> GPSQPTYPGDDAP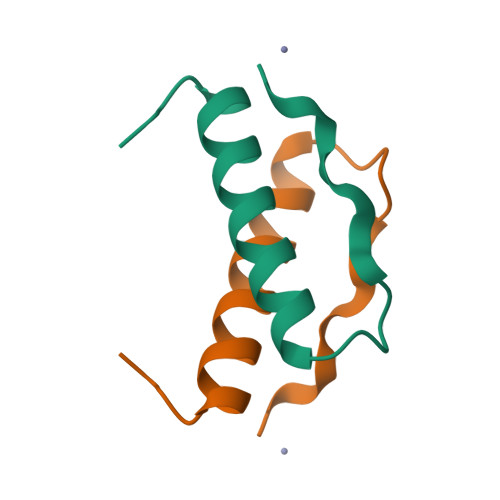VEDLIRFYDNLQQYLNVVTRHRY>SDEVRKNLMDMFRDRQAFSEHTWKMLLSVCRSWAAWCKLNNRKWFPAEPEDVRDYLLYLQARGLAVKTIQQHLGQLNMLHRRSGLPRPSDSNAVSLVMRRIRKENVDAGERAKQALAFERTDFDQVRSLMENSDRCQDIRNLAFLGIAYNTLLRIAEIARIRVKDISRTDGGRMLIHIGRTKTLVSTAGVEKALSLGVTKLVERWISVSGVADDPNNYLFCRVRKNGVAAPSATSQLSTRALEGIFEATHRLIYGAKDDSG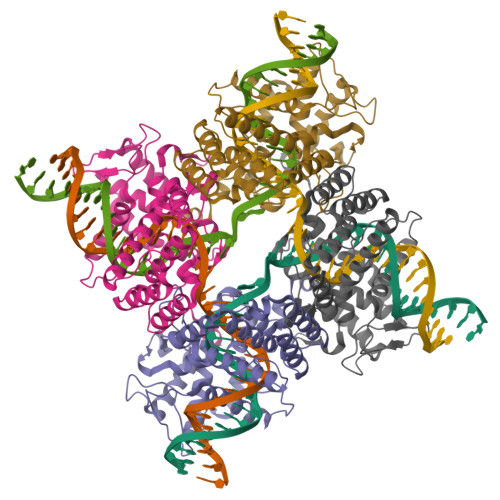QRYLAWSGHSARVGAARDMARAGVSIPEIMQAGGWTNVNIVMNYIRNLDSETGAMVRLLEDGD[2x]> METVTIEHRLGKTTLEQKPQRVVVIGVGALDAIDSFGIEPVAVSKFDGTPDYLAKYKSDKYPSAGSLFEPDFETIYTQKPDLIVIGPRASKSYDELSKIAPTIVFAAEADQGYWESTQQQWRNLGKVFAIEPAVEAKIEQVDAQFKSIMQYNQQHKSDAMLVMSSGGNLTTFGANSRFSSVYKDFGFSETVPVSKES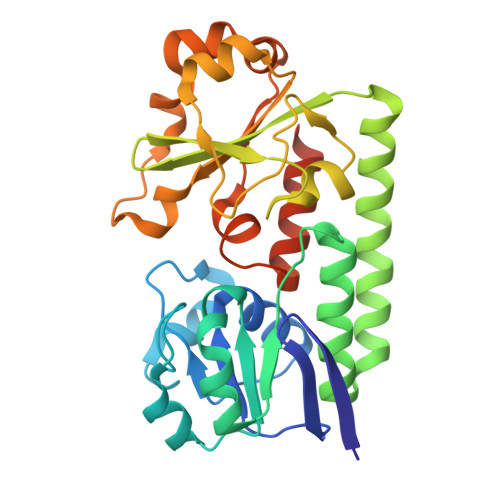SHGDLISFEYIREHNPKTLLVVDRDKVVTKGETNIRQTFENDLVKATTAYKNGHIAYLDVNAWYIAISGVKATEQMVADMKASVGMQLEHHHHHH> GAMSSIFINREYLLPDYIPDELPHREDQIRKIASILAPLYREEKPNNIFIYGLTGTGKTAVVKFVLSKLHKKFLGKFKHVYINTRQIDTPYRVLADLLESLDVKVPFTGLSIAELYRRLVKAVRDYGSQVVIVLDEIDAFVKKYNDDILYKLSRINSEVNKSKISFIGITNDVKFVDLLDPRVKSSLSEEE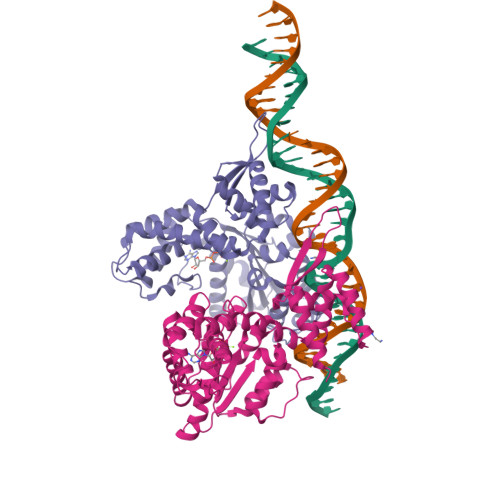IIFPPYNAEELEDILTKRAQMAFKPGVLPDNVIKLCAALAAREHGDARRALDLLRVSGEIAERMKDTKVKEEYVYMAKEEIERDRVRDIILTLPFHSKLVLMAVVSISSEENVVSTTGAVYETYLNICKKLGVEAVTQRRVSDIINELDMVGILTAKVVNRGRYGKTKEIGLAVDKNIIVRSLIESDSRFADLWS;> GAMEVIKNPKVFIDPLSVFKEIPFREDILRDAAIAIRYFVKNEVKFSNLFLGLTGTGKTFVSKYIFNEIEEVKKEDEEYKDVKQAYVNCREVGGTPQAVLSSLAGKLTGFSVPKHGINLGEYIDKIKNGTRNIRAIIYLDEVDTLVKRRGGDIVLYQLLRSDANISVIMISNDINVRDYMEPRVLSSLGPSVIFKPYDAEQLKFILSKYAEYGLIKGTYDDEILSYIAAISAKEHGDARKAVNLLFRAAQLASGGGIIRKEHVDKAIVDYEQERLIEAVKALPFHYKLALRSLIESEDVMSAHKMYTDLCNKFKQKPLSYRRFSDIISELDMFGIVKIRIINRGRAGGVKKYALVEDKEKVLRALNETFEDSISIGDFDDVGEN>MAQILPIRFQEHLQLQNLGINPANIGFSTLTMESDKFICIREKVGEQAQVVIIDMNDPSNPIRRPISADSAIMNPASKVIALKAGKTLQIFNIEMKSKMKAHTMTDDVTFWKWISLNTVALVTDNAVYHWSMEGESQPVKMFDRHSSLAGCQIINYRTDAKQKWLLLTGISAQQNRVVGAMQLYSVDRKVSQPIEGHAASFAQFKMEGNAEESTLFCFAVRGQAGGKLHIIEVGTPPTGNQPFPKKAVDVFFPPEAQNDFPVAMQISEKHDVVFLITKYGYIHLYDLETGTCIYMNRISGETIFVTAPHEATAGIIGVNRKGQVLSVCVEEENIIPYITNVLQNPDLALRMAVRNNLAGAEELFARKFNALFAQGNYSEAAKVAANAPKGILRTPDTIRRFQSVPAQPGQTSPLLQYFGILLDQGQLNKYESLELCRPVLQQGRKQLLEKWLKEDKLECSEELGDLVKSVDPTLALSVYLRANVPNKVIQCFAETGQVQKIVLYAKKVGYTPDWIFLLRNVMRISPDQGQQFAQMLVQDEEPLADITQIVDVFMEYNLIQQCTAFLLDALKNNRPSEGPLQTRLLEMNLMHAPQVADAILGNQMFTHYDRAHIAQLCEKAGLLQRALEHFTDLYDIKRAVVHTHLLNPEWLVNYFGSLSVEDSLECLRAMLSANIRQNLQICVQVASKYHEQLSTQSLIELFESFKSFEGLFYFLGSIVNFSQDPDVHFKYIQAACKTGQIKEVERICRESNCYDPERVKNFLKEAKLTDQLPLIIVCDRFDFVHDLVLYLYRNNLQKYIEIYVQKVNPSRLPVVIGGLLDVDCSEDVIKNLILVVRGQFSTDELVAEVEKRNRLKLLLPWLEARIHEGCEEPATHNALAKIYIDSNNNPERFLRENPYYDSRVVGKYCEKRDPHLACVAYERGQCDLELINVCNENSLFKSLSRYLVRRKDPELWGSVLLESNPYRRPLIDQVVQTALSETQDPEEVSVTVKAFMTADLPNELIELLEKIVLDNSVFSEHRNLQNLLILTAIKADRTRVMEYINRLDNYDAPDIANIAISNELFEEAFAIFRKFDVNTSAVQVLIEHIGNLDRAYEFAERCNEPAVWSQLAKAQLQKGMVKEAIDSYIKADDPSSYMEVVQAANTSGNWEELVKYLQMARKKARESYVETELIFALAKTNRLAELEEFINGPNNAHIQQVGDRCYDEKMYDAAKLLYNNVSNFGRLASTLVHLGEYQAAVDGARKANSTRTWKEVCFACVDGKEFRLAQMC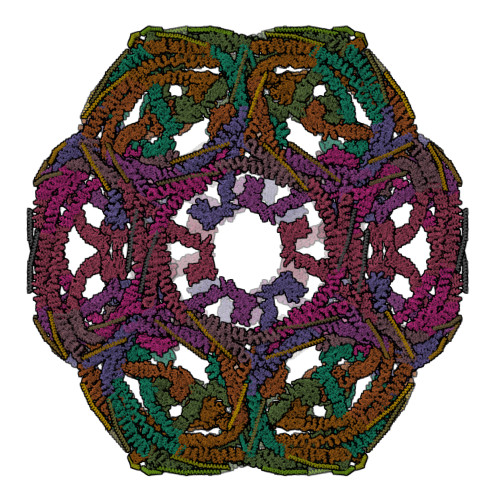GLHIVVHADELEELINYYQDRGYFEELITMLEAALGLERAHMGMFTELAILYSKFKPQKMREHLELFWSRVNIPKVLRAAEQAHLWAELVFLYDKYEEYDNAIITMMNHPTDAWKEGQFKDIITKVANVELYYRAIQFYLEFKPLLLNDLLMVLSPRLDHTRAVNYFSKVKQLPLVKPYLRSVQNHNNKSVNESLNNLFITEEDYQALRTSIDAYDNFDNISLAQRLEKHELIEFRRIAAYLFKGNNRWKQSVELCKKDSLYKDAMQYASESKDTELAEELLQWFLQEEKRECFGACLFTCYDLLRPDVVLETAWRHNIMDFAMPYFIQVMKEYLTKVDKLDASESLRKEEEQATETQ[9x];>[9x]VDRLQSEPESIRKWREEQTERLEALDANSRKQEAEWKEKAIKELDEWYARQDEQLQKTKANNRVADEAFY> MAKLTALTLLGMGLALFDRQKSSFQTRFNVHREVTPVELPNCNLVK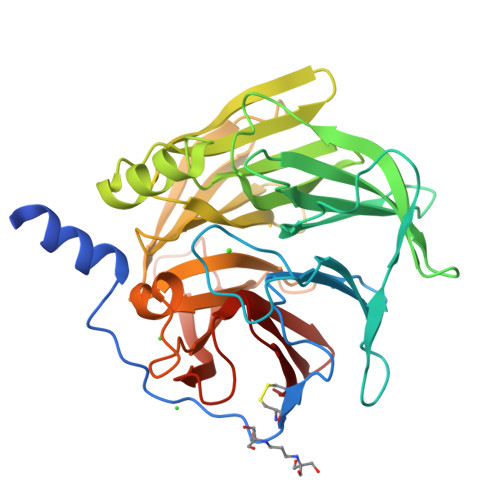GIDNGSEDLEILPNGLAFISSGGKYPGIMSFDPDKSGKILLMDLNEKEPAVSELEIIGNTLDISSFNPHGISTFIDDDNTVYLLVVNRPGSSSTVEVFKFQEEEKSLLHLKTIRHKLLPSVNDIVAVGPEHFYATNDHYFIDPYLKSWEMHLGLAWSFVTYYSPNDVRVVAEGFDSANGINISPDGKYVYIAELLAHKIHVYEKHANWTLTPLRVLSFDTLVDNISVDPVTGDLWVGCHPNGMRIFFYDAENPPGSEVLRIQDILSEEPKVTVVYAENGTVLQGSSVAAVYKGKLLIGTVFHKALYCDL> MEVLFEAKVGDITLKLAQGDITQYPAKAIVNAANKR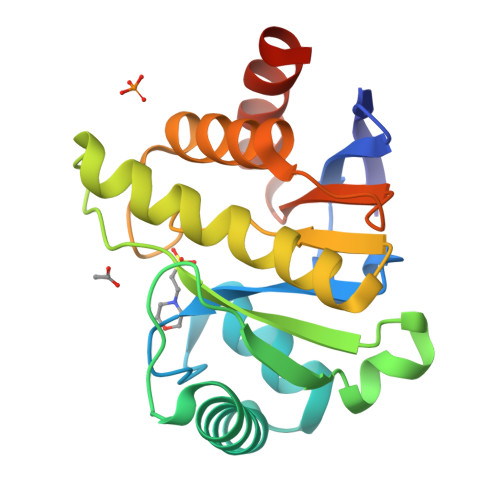LEHGGGVAYAIAKACAGDAGLYTEISKKAMREQFGRDYIDHGEVVVTPAMNLEERGIKYVFHTVGPICSGMWSEELKEKLYKAFLGPLEKAEEMGVESIAFPAVSAGIYGCDAEKVVETSLEAVKNFKGSAVKEVAEVHGARKSAEVALKVFERSLEHHHHHH>GVSKTFKDKCASTTAKLVQSVQLVNISSDVNKDSKGIYISSSAGKTWFIPGGQYYPDNYLSNEMRKIAMAA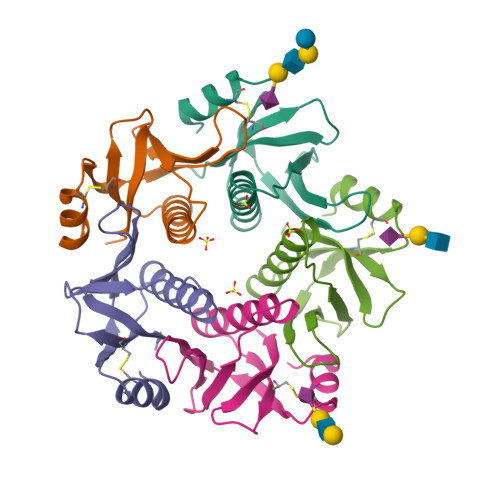VLSNVRVNLCASEAYTPNHVWAIELAPHHHHHH[10x]>GPLGSNRKRLPSYLKPGSAVEISSDEIGFRGSWYMGKVITIPSSSDKDSVKCQVEYTTLFFDKEGTKPLKEVVDMSQLRPPAPPMSEIEKKKKIVVGEEVDAFYNDGWWEGDVTEVLDDGKFSVFFRSSKEQIRFRKDELRFHRE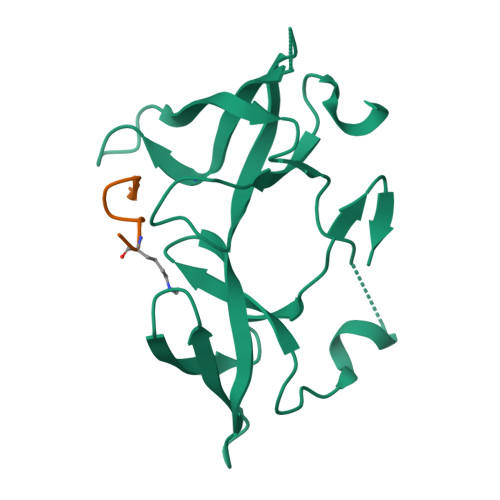WVDGAWK[4x];>ARTKQTARKST[4x]Neprilysin, or neutral endopeptidase (NEP), is an integral type II membrane-bound zinc-dependent peptidase of approximately 750 amino acid residues that degrades a number of physiological peptides that are involved in processes such as blood pressure regulation and nociception. NEP is composed of an ectodomain, which contains the catalytic site and belongs to the M13 family of peptidases/proteases, a transmembrane domain and a short intracellular domain. The structure of the ectodomain is composed of two largely α-helical domains (domains 1 and 2) that are arranged to form a central spherical water-filled core that contains the active site of the enzyme. The larger N-terminal domain (domain 1), which is structurally related to the bacterial protease thermolysin, contains a single zinc atom that is critical for peptidase activity and is coordinated by His and Glu residues.

The overall structure of the double mutant NEP is similar to wild-type NEP, with two domains which are connected by three interdomain linker segments, together enclosing a large water filled cavity. The second mutated residue Val399 is at a distance of 20 Å from Lys714, located in the smaller domain (domain 2) at the surface of the protein at the interface between the two domains. The interdomain distance, as measured by Cα-Cα distance from residue Val399 in domain 2 to e. g. residue Arg698 in domain 1, increases by more than 2 Å (from 5.9 Å to 8.4 Å in wild-type NEP and NEPv, respectively). Furthermore Lys714 limits the conformational flexibility of Trp693 and thereby reduces the plasticity and size of the S1’ pocket. The overall binding mode of phosphoramidon in the NEP double mutant is similar to that observed in wild-type. The C-terminal extension of the phosphoramidon binds differently. While the phosphoramidon tryptophan pyrrole retains the interaction with Val541 O and the stacking interaction with Phe106, the positions of the phosphoramidon tryptophan and Phe106 side chain moieties are interchanged. Large ligand induced flexibility of amino acid side chains is observed in the substrate binding site, with particularly Trp693 functioning as a switch between the S1’ and S2’ pockets in wild-type NEP; (P1’ and P2’ dependency shown in Oefner et al.,, Glossop et al.,). In the crystal structure of the NEPv presented here, the two mutations have reduced the substrate binding sites S1’ and S2’ as well as decreased the binding site plasticity.

> HHHHHHHHHHYDDGICKSSDCIKSAARLIQNMDATTEPCTDFFKYACGGWLKRNVIPETSSRYGNFDILRDELEVVLKDVLQEPKTEDIVAVQKAKALYRSCINESAIDSRGGEPLLKLLPDIYGWPVATENWEQKYGASWTAEKAIAQLNSKYGKKVLINLFVGTDDKNSVNHVIHIDQPRLGLPSRDYYECTGIYKEACTAYVDFMISVARLIRQEERLPIDENQLALEMNKVMELEKEIANATAKPEDRNDPMLLYNKMTLAQIQNNFSLEINGKPFSWLNFTNEIMSTVNISITNEEDVVVYAPEYLTKLKPILTKYSARDLQNLMSWRFIMDLVSSLSRTYKESRNAFRKALYVTTSETATWRRCANYVNGNMENAVGRLYVEAAFAGESKHVVEDLIAQIREVFIQTLDDLTWMDAETKKRAEEKALAIKERIGYPDDIVSNDNKLNNEYLELNYKEDEYFENIIQNLKFSQSKQLKKLREKVDKDEWISGAAVVNAFYSSGRNQIVFPAGILQPPFFSAQQSNSLNYGGIGMVIGHEITHGFDDNGRNFNKDGDLVDWWTQQSASNFKEQSQCMVYQYGNFSWDLAGGQHLNGINTLGENIADNGGLGQAYRAYQNYIKKNGEEKLLPGLDLNHKQLFFLNFAQVWCGTYRPEYAVNSIKTDVHSPKNFRIIGTLQNSAEFSEAFHCRKNSYMNPEKKCRVW>MAHHHHHHVDDDDKVAAQKKKAQDEYGAASITILEGLEAVRKRPGMYIGSTGERGLHHLIWEVVDNAVDEAMAGYATTVNVVLLEDGGVEVADDGRGIPVATHASGIPTVDVVMTQLHAGGKFDSDAYAISGGLHGVGVSVVNALSTRLEVEIKRDGYEWSQVYEKSEPLGLKQGAPTKKTGSTVRFWADPAVFETTEYDFETVARRLQEMAFLNKGLTINLTDERVTQDEVVDEVVSDVAEAPKSASERAAESTAPHKVKSRTFHYPGGLVDFVKHINRTKNAIHSSIVDFSGKGTGHEVEIAMQWNAGYSESVHTFANTINTHEGGTHEEGFRSALTSVVNKYAKDRKLLKDKDPNLTGDDIREGLAAVISVKVSEPQFEGQTKTKLGNTEVKSFVQKVCNEQLTHWFEANPTDAKVVVNKAV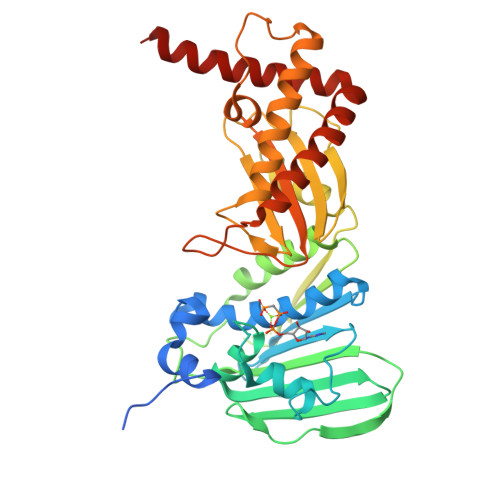SSAQARIAARKARELVR[6x]> GAMGSLFNSEEDVVKMSPLPTVENQFTPTTAWSTSVGSGIGNFYSNLHPALADNVVYAADRAGLVKALNADDGKEIWSVSLAEKDGWFSKEPALLSGGVTVSGGHVYIGSEKAQVYALNTSDGTVAWQTKVAGEALSRPVVSDGLVLIHTSNGQLQ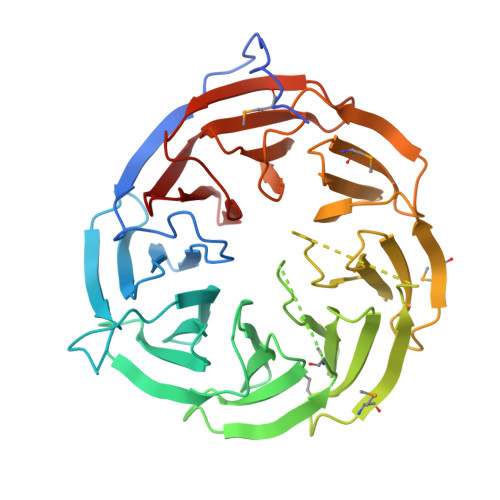ALNEADGAVKWTVNLDMPSLSLRGESAPTTAFGAAVVGGDNGRVSAVLMEQGQMIWQQRISQATGSTEIDRLSDVDTTPVVVNGVVFALAYNGNLTALDLRSGQIMWKRELGSVNDFIVDGNRIYLVDQNDRVMALTIDGGVTLWTQSDLLHRLLTSPVLYNGNLVVGDSEGYLHWINVEDGRFVAQQKVDSSGFQTEPVAADGKLLIQAKDGTVYSITR> MAESTTLETIEIHPITFPPEVLARISPELSLQRHLSLGIRPCLRKYEEFRDVAIENNTLSRYADAGNIDTKNNILGSNVLKSGKTIVITSITGGIIEETSAAIKDLDDFGEEELFEVTKEEDIIANYASVYPVVEVERGRVGACTDEEMTISQKLHDSILHSRILPKKALKVKAGVRSANEDGTFS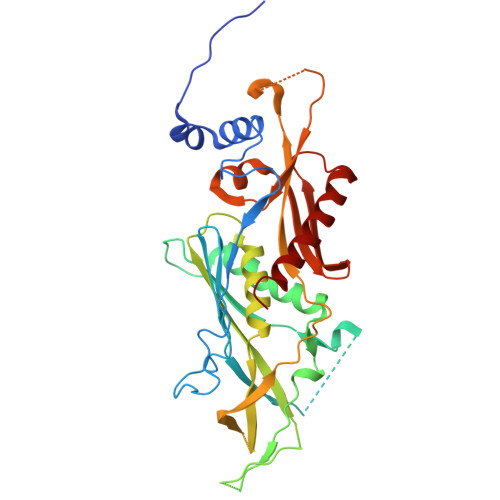VLYPDELEDDTLNETNLKMKRKWSYVLYAKIVVLSRTGPVFDLCWNSLMYALQSVKLPRAFIDERASDLRMTIRTRGRSATIRETYEIICDQTKSVPLMINAKNIAFASNYGIVELDPECQLQNSDNSEEEEVDIDMDKLNTVLIADLDTEAEETSIHSTISILAAPSGNYKQLTLVGGGAKITPEMIKRSLLLSRVRADDLSTRFNI> EGPPPAM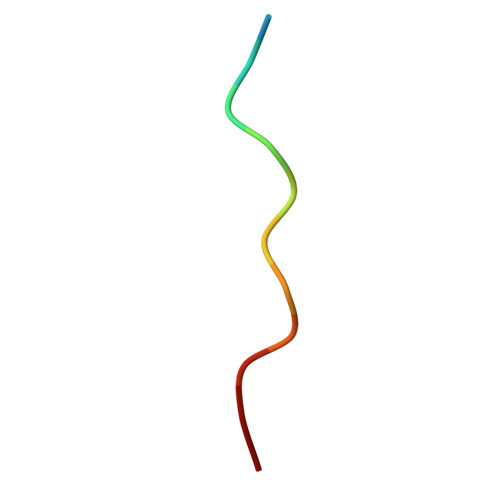PARPT> MRHDGRQHDELRPITFDLDFISHPEGSVLITAGNTKVICNASVEDRVPPFLRGGGKGWITAEYSMLPQATNQQTIQESSKGKISGRTMEIQRLIGRALRAVVDLEKLGERTIWIDCDVIQADGGTRTASITGAFLA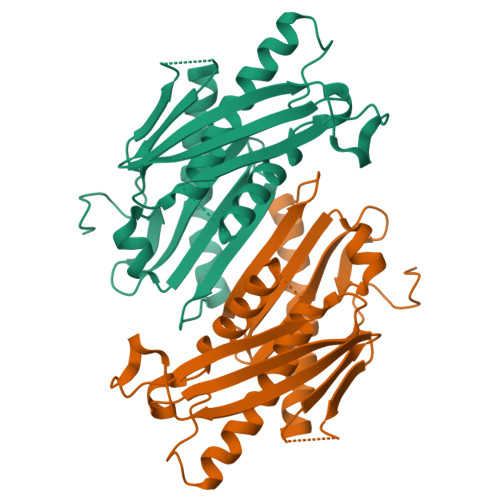MAIAIGKLIKAGTIKTNPITDFLAAISVGIDKEQGILLDLNYEEDSSAEVDMNVIMTGSGRFVELQGTGEEATFSREDLNGLLGLAEKGIQELIDKQKEVLGDSLPELK> ALANTFLVKEDSKNVTAYTPFATPITDSKSDLVSLAQLDSSYQIADQTIHNTNLFVLFKSRDVKVKYESSGSNNISFDSTSQGEKPSYVVEFTNSTNIGIKWTMVKKYQLDVPNVSSDMNQVLKNLILEQPLTKYTLNS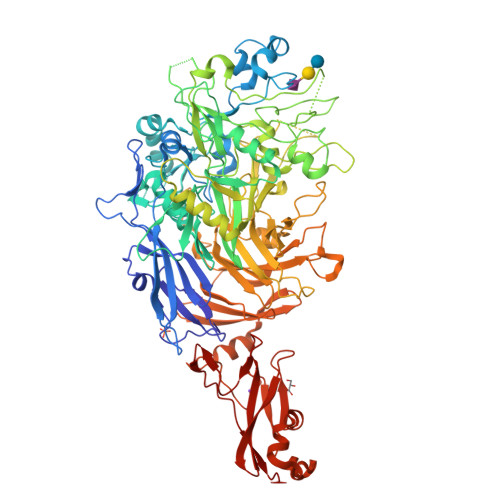SLAKEKGKTQREVHLGSGQANQWTSQRNQHDLNNNPSPNASTGFKLTTGNAYRKLSESWPIYEPIDGTKQGKGKDSSGWSSTEENEAKNDAPSVSGGGSSSGTFNKYLNTKQALESIGILFDDQTPRNVITQLYYASTSKLAVTNNHIVVMGNSFLPSMWYWVVERSAQENASNKPTWFANTNLDWGEDKQKQFVENQLGYKETTSTNSHNFHSKSFTQPAYLISGIDSVNDQIIFSGFKAGSVGYDSSSSSSSSSSSTKDQALAWSTTTSLDSKTGYKDLVTNDTGLNGPINGSFSIQDTFSFVVPYSGNHTNNGTTGPIKTAYPVKKDQKSTVKINSLINATPLNSYGDEGIGVFDALGLNYNFKSNQERLPSRTDQIFVYGIVSPNELRSAKSSADSTGSDTKVNWSNTQSRYLPVPYNYSEGIIDADGFKRPENRGASVTTFSGLKSIAPDGFANSIANFSVGLKAGIDPNPVMSGKKANYGAVVLTRGGVVRLNFNPGNDSLLSTTDNNIAPISFSFTPFTAAESAVDLTTFKEVTYNQESGLWSYIFDSSLKPSHDGKQTPVTDNMGFSVITVSRTGIELNQDQATTTLDVAPSALAVQSGIQSTTQTLTGVLPLSEEFSAVIAKDSDQNKIDIYKNNNGLFEIDTQLSNSVATNNGGLAPSYTENRVDAWGKVEFADNSVLQARNLVDKTVDEIINTPEILNSFFRFTPAFEDQKATLVATKQSDTSLSVSPRIQFLDGNFYDLNSTIAGVPLNIGFPSRVFAGFAALPA>MGSSHHHHHHHHHHSSGLVPRGSHMSAIGTVFKEHVKNFYLIQRLAQFQVKIINHSNYLGVAWELINPVMQIMVYWMVFGLGIRSNAPIHGVPFVYWLLVGISMWFFINQGILEGTKAITQKFNQVSKMNFPLSIIPTYIVTSRFYGHLGLLLLVIIACMFTGIYPSIHIIQLLIYVPFCFFLTASVTLLTSTLGVLVRDTQMLMQAILRILFYFSPILWLPKNHGISGLIHEMMKYNPVYFIAESYRAAILYHEWYFMDHWKLMLYNFGIVAIFFAIGAYLHMKYRDQFADFL[2x];>[2x]MNVSVNIKNVTKEYRIYRTNKERMKDALIPKHKNKTFFALDDISLKAYEGDVIGLVGINGSGKSTLSNIIGGSLSPTVGKVDRNGEVSVIAISAGLSGQLTGIENIEFKMLCMGFKRKEIKAMTPKIIEFSELGEFIYQPVKKYSSGMRAKLGFSINITVNPDILVIDEALSVGDQTFAQKCLDKIYEFKEQNKTIFFVSHNLGQVRQFCTKIAWIEGGKLKDYGELDDVLPKYEAFLNDFKKKSKAEQKEFRNKLDESRFVIK

Wall teichoic acid (WTA) is a polyol phosphate polymer that covalently decorates peptidoglycan of gram-positive bacteria, including Staphylococcus aureus. Central to WTA biosynthesis is flipping of lipid-linked precursors across the cell membrane by TarGH, a type V ABC transporter. TarGH is a heterotetramer composed of two TarG polytopic transmembrane domains (TMD) and two TarH nucleotide binding domains (NBD). Like other ABC transporters, TarGH uses the energy derived from the ATP hydrolysis cycle in the NBDs to drive substrate transport across the membrane via the TMDs.

To investigate if these differences were a result of targocil-II binding or the choice of ATP analogue, we determined structures of TarGH produced in L. lactis in complex with ATPγS alone and with targocil-II. The structure in complex with ATPγS alone (2.9 Å resolution) is near identical to the E. coli produced protein (RMSD 0.58 Å and 0.52 Å across TarH and TarG Cα-atoms, respectively). The first, in complex with ATPγS, shows the TarH D-loop in a conformation (D-loopOFF) that appears non-competent for ATP hydrolysis. We suggest that the D-loopOFF state in the absence of substrate could provide a mechanism to minimise spurious waste of ATP when not needed for WTA polymer flipping.> LDLFVSPLGRVEGDLDVRVTINDGVVTSAWTEAAMFRGFEIILRGKDPQAGLIVCPRICGICGGSHLYKSAYALDTAWRTHMPPNATLIRNICQACETLQSIPRYFYALFAIDLTNKNYAKSKLYDEAVRRFAPYVGTSYQPGVVLSAKPVEVYAIFGGQWPHSSFMVPGGVMSAPTLSDVTRAIAILEHWNDNWLEKQWLGCSVDRWLENKTWNDVLAWVDENESQYNSDCGFFIRYCLDVGLDKYGQGVGNYLATGTYFEPSLYENPTIEGRNAALIGRSGVFADGRYFEFDQANVTEDVTHSFYEGNRPLHPFEGETIPVNPED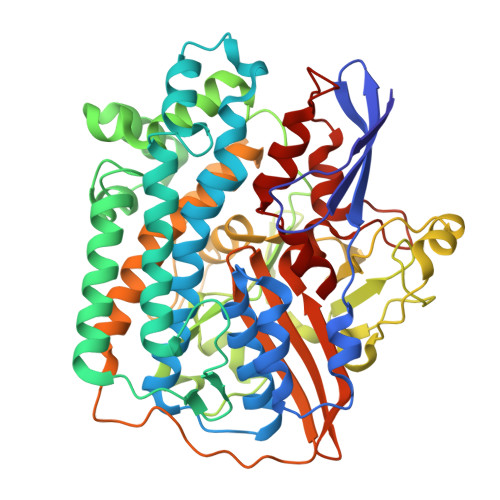GRRQGKYSWAKSPRYAVPGLGNVPLETGPLARRMAASAPDAETHQDDDPLFADIYNAIGPSVMVRQLARMHEGPKYYKWVRQWLDDLELKESFYTKPVEYAEGKGFGSTEAARGALSDWIVIEDSKIKNYQVVTPTAWNIGPRDASEVLGPIEQALVGSPIVDAEDPVELGHVARSFDSCLVCTVH The human proteome comprises 266 human PDZ (PSD95/DLG1/ZO1) domains 16 and about 4000 putative PBMs, defining a network of one million potential interactions. PBMs are mostly (though not exclusively) C-terminal, with their COO- implicated in binding, and are classified based on position −2, being respectively Ser/Thr, hydrophobic or acidic in classes 1, 2, and 3 17,18. PDZ-PBM interactions are rather transient and promiscuous. Viral proteins bearing functional PBMs are found notably in HPV and HTLV oncoviruses as well as in HBV, WNV and coronaviruses including MERS or SARS-CoV213,15,23–26.

The logos of PDZ domains SNTB1 and MAGI1_2 indicate preferences for x-R-E-T-x-V-COO- and R-x-E-T-x-V-COO-, respectively. The oncoviral PBM of HPV35 E6 satisfies both consensus requirements hence recognizes both PDZ domains. The structures of HPV35 E6 PBM bound to both SNTB1 and MAGI1_2 resolve their logo differences by revealing the distinctive contributions of Arg residues at p-4 and p-5 of HPV35 E6 in the two complexes. B The affinity-weighted specificity logo of SNTB1 PDZ matches well with HPV35 E6 PBM at positions p0, p-2, p-3 and p-4, which display favorable contacts in the crystal structure of the SNTB1/HPV35 E6 complex. Accordingly, HPV35 E6 binds stronger to MAGI1-2 than to SNTB1.

> GSHMGSNQKRGVKVLKQELGGLGISIKGGKENKMPILISKIFKGLAADQTQALYVGDAILSVNGADLRDATHDEAVQALKRAGKEVLLEVKYMREGSAYGSVKAYTNFDAERDALNIETAIKTKGVDEVTIVNILTNRSNEQRQDIAFAYQRRTKKELASALKSALSGHLETVILGLLKTPAQYDASELKASMKGLGTDEDSLIEIICSRTNQELQEINRVYKEMYKTDLEKDIISDTSGDFRKLMVALAKGRRAEDGSVIDYELIDQDARDLYDAGVKRKGTDVPKWISIMTERSVPHLQKVFDRYKSYSPYDMLESIRKEVKGDLENAFLNLVQCIQNKPLYFADRLYDSMKGKGTRDKVLIRIMVSRSEVDMLKIRSEFKRKYGKSLYYYIQQDTKGDYQKALLYLCGGDD;> TDDSKPTRRETEV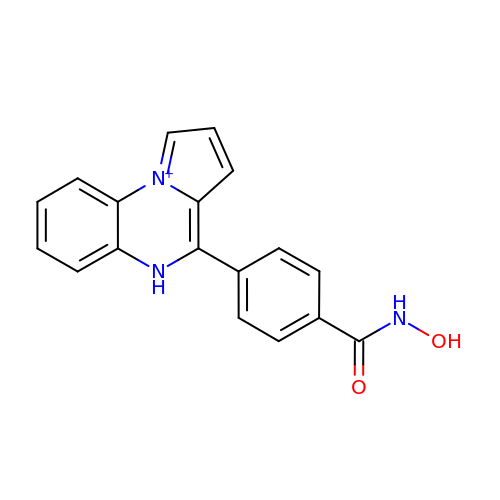~{N}-oxidanyl-4-(5~{H}-pyrrolo[1,2-a]quinoxalin-4-yl)benzamide | C18 H14 N3 O2 | UIYKYEMVZGDMRC-UHFFFAOYSA-O> GIDPFTNPRTVKITASSEETSGENAPASFASDGDMNTFWH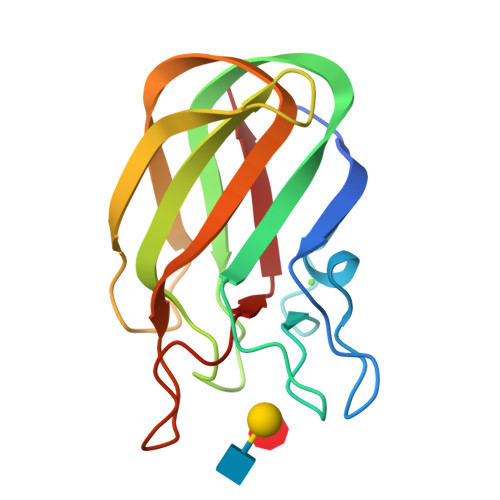SKWSSPAHEGPHHLTLELDNVYEINKVKYAPRQDSKNGRITGYKVSVSLDGENFTEVKTGTLEDNAAIKFIEFDSVDAKYVRLDVTDSVSDQANGRGKFATAAEVNVHG>GSMELRVGNRYRLGRKIGSGSFGDIYLGTDIAAGEEVAIKLECVKTKHPQLHIESKIYKMMQGGVGIPTIRWCGAEGDYNVMVMELLGPSLEDLFNFCSRKFSLKTVLLLADQMISRIEYIHSKNFIHRDVKPDNFLMGLGKKGNLVYIIDFGLAKKYRDARTHQHIPY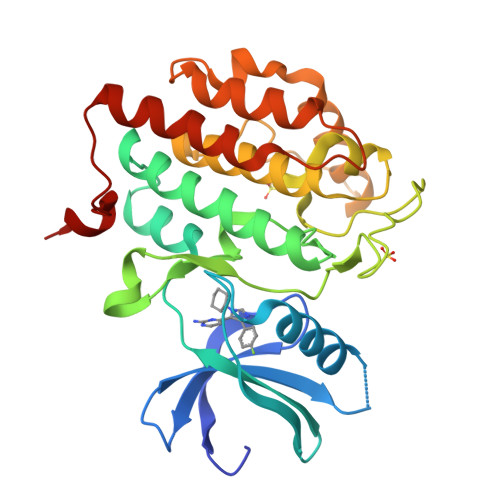RENKNLTGTARYASINTHLGIEQSRRDDLESLGYVLMYFNLGSLPWQGLKAATKRQKYERISEKKMSTPIEVLCKGYPSEFATYLNFCRSLRFDDKPDYSYLRQLFRNLFHRQGFSYDYVFDWNMLK[4x]> QS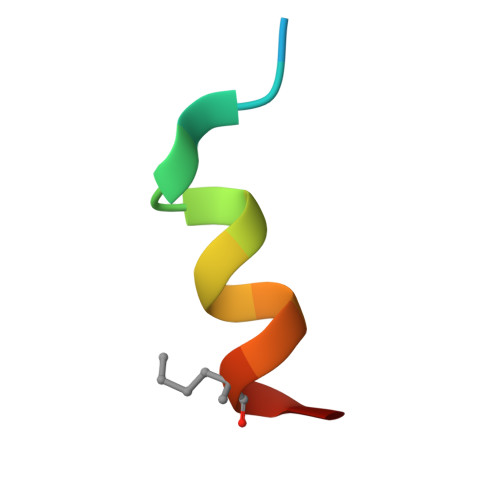QQTFXNLWRLLLQNX> DRVYIHPFHLLYYSKSTCAQLENPSVETLPEPTFEPVPIQAKTSPVDEKTLRDKLVLATEKLEAEDRQRAAQ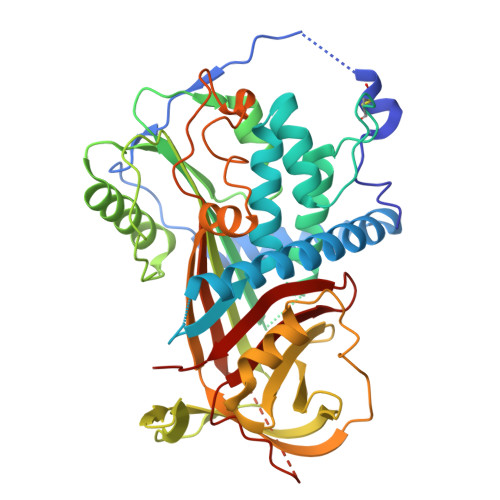VAMIANFMGFRMYKMLSEARGVASGAVLSPPALFGTLVSFYLGSLDPTASQLQVLLGVPVKEGDCTSRLDGHKVLTALQAVQGLLVTQGGSSSQTPLLQSTVVGLFTAPGLRLKQPFVESLGPFTPAIFPRSLDLSTDPVLAAQKINRFVQAVTGWKMNLPLEGVSTDSTLFFNTYVHFQGKMRGFSQLTGLHEFWVDNSTSVSVPMLSGTGNFQHWSDAQNNFSVTRVPLGESVTLLLIQPQCASDLDRVEVLVFQHDFLTWIKNPPPRAIRLTLPQLEIRGSYNLQDLLAQAKLSTLLGAEANLGKMGDTNPRVGEVLNSILLELQAGEEEQPTESAQQPGSPEVLDVTLSSPFLFAIYERDSGALHFLGRVDNPQNVV>AQPGRKLGYAILGLGYYATRIIMPRFAECEHSRLAALVSGTPEKLKTYGEQYGIPETHRYSYETFDRIIDNPDVDIVYVITPNSLHRPFTERAARAGKHVMCEKPMANTVADCEAMIAACKKAGRKLMIGYRSRFQAHNIEAIKLVRDGALGPVRTVVTDHGFTIGDPKQWRLNRALAGGGSLMDIGIYSLNAARYLTGEEPVAVNAVESTDRSDPRFGEVEDIINFQLLFPSGATANCVSAYSVNCNRYRVSGPKGWVEIDPATSYQGQAMRAQLGGPPAPREPAPQPKNQFSAQLDHLSECILTGREPIVGGDDGLKDLRVIEAIYRA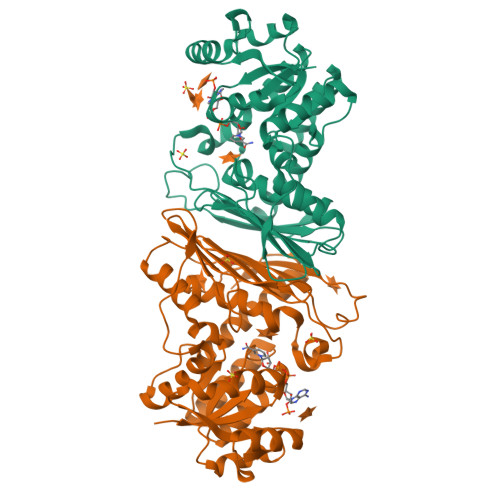AREGRTVKL[6x]>GSAKDPMHNFTYWNPTKLIFGRGEV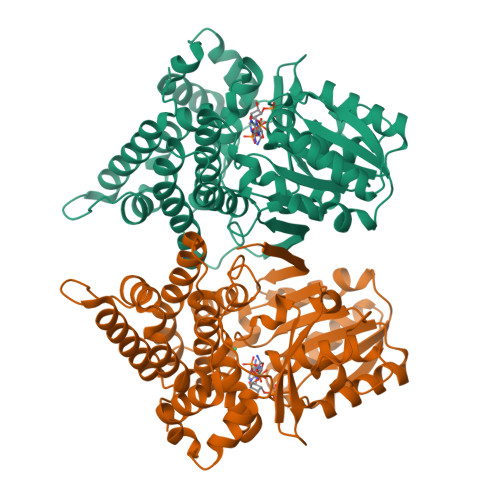ERLPEELKSYGKNVLLVYGGGSIKRSGLYDQVIEQLNKAGVTVHELAGVEPNPRVSTVNKGVALCKEHHIDFLLAVGGGSVIDCTKAIAAGAKYDGDAWDIVTKKHQPKDALPFGTVLTLAATGSEMNSGSVITNWETKEKYGWGSPLVFPKFSILDPVNTFTVPKNHTIYGMVDMMSHVFEQYFHHVSNTPYQDRMCESLLRTVIETAPKLINDLENYELRETILYTGTIALNGMLSMGARGDWATHNIEHAVSAVYDIPHAGGLAILFPNWMRHTLSENPARMKQLAVRVFGVEEAGKTDKEVALEGIDKLSAFWTSLGAPNRLADYDINDEQLDTIADKAMANGTFGQFKSLNKEDVLAILKASL[4x]> NSK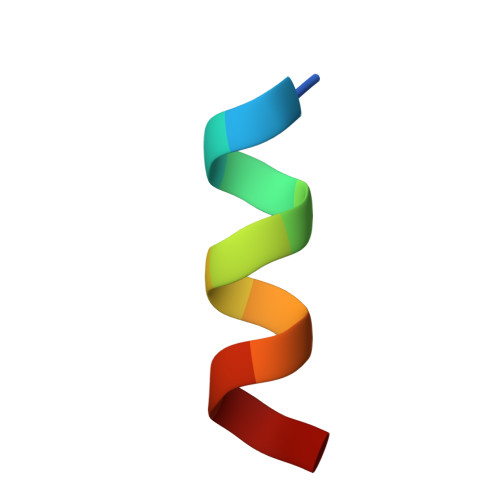LLSLLRSKT> MRHTIPFF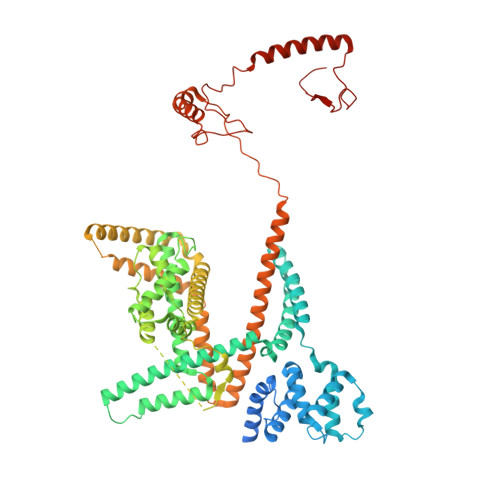RRSAFVPAPGSSLLNPRSQRAKVRRMVAAQKAQGENFERQALYAELGGSPSARAPRSKGERSKEATRRVGCEVAERAKHMTDAEWEGVPVDEKHAFAKYMHKVLQEHPTETTEQQRRRYFETTMADVFELDPRKTVRDEYERVKLGLPVHLKNPQYSLGVSQAVYDAADASLFDPENVHRLENAMTHVKQVFADYVHKKREGVSTEAERRMLANLTAELNLETQKHLANMFKYAEMRLRQVKLEERHHQLAEIERLRRMAQQRGGVKGRKGGSRKMSRMERLKRVINRAVGLDIAVAETVLTEMQAQEEFLQFCEVFARLTLGSGFKHTGKDENLSAYIESLRKLYSMDAATLSTLDVVQYYSSKEGAHPVDWAKRWYERALLLPLQSTPEYQKLLQIQQRDESTVKHIKETAGTGHAFACEAEAEVARIKTQKVVNLVEKMFMDPKDKRLESLHEKRLRYLAHMQMERQIRCVRENAKLFDGVENMPEAAQCRELYEKIMEKKTAQCNMTSPPEGEGSAIQSAKTEGDHCEVGPGMFNVYDDAEASSLFEKIREITLRVIRDRRVQSAAATKARMLNRIIRSLKGGERSIAEELRALHQQRKEKMTMRILGIIENDVKTEMEWLQNMEEAERPPLLPIPENMSYVSAADVQAWRELREDDERKAANPFERRRRTFQPELLGQAWSVPNKPLLFWGTGVSAVQQALRHVAEDAERKRQGLLLAPPYPCAENPWGWRLAKDILDDNN> KPQIITQPETTMAMVGKDIRFTCSAASSSSSPMTFAWKKDNEVLTNA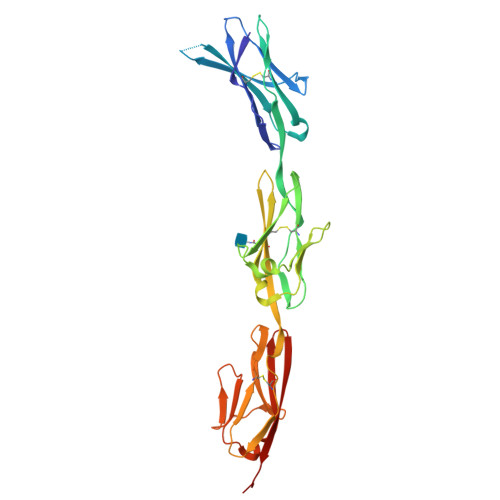DMENFVHVHAQDGEVMEYTTILHLRQVTFGHEGRYQCVITNHFGSTYSHKARLTVNVLPSFTKTPHDITIRTTTMARLECAATGHPNPQIAWQKDGGTDFPAARERRMHVMPDDDVFFITDVKIDDAGVYSCTAQNSAGSISANATLTVLETPSLVVPLEDRVVSVGETVALQCKATGNPPPRITWFKGDRPLSLTERHHLTPDNQLLVVQNVVAEDAGRYTCEMSNTLGTERAHSQLSVLLENLY> GSNEKIRSQSVLNTLETFFIKENHYDMQREESSIVN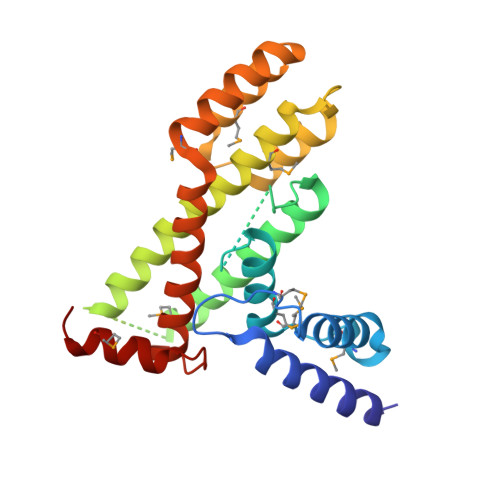ACLRYLGYSKSMCHEKMPIFMDIAFIEYCFNLSLDPSSFQNLPITQTQPDSQQILWEYSLISNALERLENIELERQNCMREDGLVKYTNELLLNKETLNNEALKLYSCAKAGICRWMAFHFLEQEPIDHINFTKFLQDWGSHNEKEMEALQRLSKHKIRKRLIYVSQHKKKMPWSKFNSVLSRYIQCTKLQLEVFCDYDFKQREIVKMLTSNIN> GSHMASQPRVIERPRLARFLADDIKAQRVAVEDAVDRSVVTIRGDELFASASASVR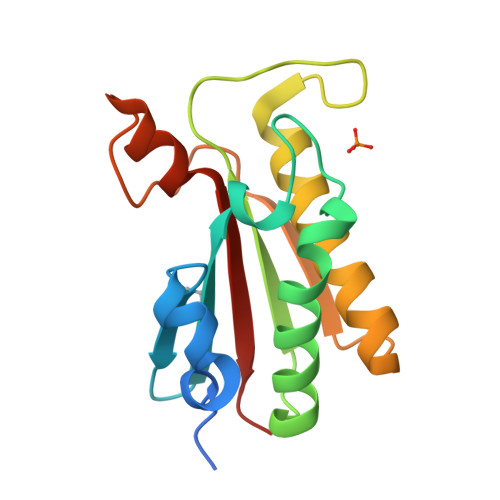DEFQPLLLRIADALRKVKGQVLVTGHSDNRPIATLRYPSNWKLSQARAQEVADLLGATTGDAGRFTAEGRSDTEPVATNASAEGRARNRRVEITVFAEGAQ> MNNNKAEADTSSSMADPETRPTYTTHHLAIPSGVTQDEFDELKQSVVEFHTYQLSQAQCSSLLAQRIRAPNDVVWSIVRRFDQPQTYKHFIKSCSVSDNFTMAVGSTRDVNVISGLPAATSTERLDILDDDRQVTGFSIIGGEHRLRNYRSVTSVHGFNRDGAICTVVLESYVVDVPEGNTEEDTRLFADTVVKLNLQKLVSVAESQVI;> RSVYELDCIPLWGVVSIQGNRSEMEDAFAVSPHFLKLPIKMLMGDHEGMSPSATHLTGHFFGVYDGHGGHKVADYCRDRLHFALAEEIERIKDELCKRNTGEGRQVQWDKVFTSCFLTVDGEIEGKIGRAVVGSSDKVLEAVASETVGSTAVVALVCSSHIVVSNCGDSRAVLFRGKEAMPLSVDHKPDREDEYARIENAGGKVIQWQGARVFGVLAMSRSIGDRYLKPYVIPEPEVTFMPRSREDECLILASDGLWDVMNNQEVCEIARRRILMWHKKNGAPPLAERGKGIDPACQAAADYLSMLALQKGSKDNISIIVIDLKAQRKFKTRT

Enhanced ABA levels elicited in response to drought are perceived by the PYR/PYL/RCAR family of ABA receptors and the clade A subfamily of protein phosphatases type 2C (PP2Cs), which act as necessary ABA co-receptors in ternary complexes. In the resting state, PYLR/PYL/RCAR receptors display an open ABA binding cavity flanked by two highly conserved loops, named as gate/CL2/β3-β4 loop and latch/CL3/β5-β6 loop. Specifically, both gate and latch loops define a surface that enables the receptor to dock into the PP2C active site. The formation of receptor-ABA-phosphatase complexes causes the dissociation of different PP2C-SnRK2 complexes and abolishes PP2C-mediated inhibition of the SnRK2s, triggering ABA response.

For instance, quinabactin (QB), also known as AM1, preferentially activates ABA dimeric receptors, whereas pyrabactin is a potent agonist for PYR1 but has antagonist effect on PYL2 (53). As a first step to improve binding of SB to CsPYL1, we determined and compared the crystal structure of CsPYL1-SB-HAB1 and CsPYL1-QB-HAB1 complexes. The gate and latch loops of CsPYL1 display a closed conformation that fits into the active site of the HAB1 phosphatase. Both ternary complexes yield isomorphous crystals whose molecular structure was almost identical to the previously reported CsPYL1-ABA-HAB1 complex. SB and QB display a “U”-shaped conformation into the ligand-binding pocket of the receptor. However, superimposition of the structures of the CsPYL1-SB-HAB1 and CsPYL1-QB-HAB1 ternary complexes reveals a shallower insertion of SB in the ABA binding pocket with respect to that observed for QB. This may be explained by the different orientation in SB and QB of the SO2 group, which contains one oxygen atom that shows similar position in both compounds and interacts through a water bridge with both Asn196 and the backbone carbonyl of His89, whereas the other oxygen is located in different position in SB and QB. Thus, in the QB complex, this latter oxygen forms a hydrogen bond with Arg108, whereas in the SB complex it produces steric hindrance with the Val110 side chain of CsPYL1. Despite this major difference, QB and SB maintain otherwise a similar network of hydrogen bond interactions in the ABA binding pocket. These include the hydrogen bonds linking the sulfonamide NH to Glu123 side chain, the SO2 group to a conserved water molecule described above, and the hydrogen bond network forming the “Trp lock”.> ETGFKCFTCEKAADNYECNRWAPDIYCPRETRYCYTQHTMEVTGNSISVTKRCVPLEECLSTGCR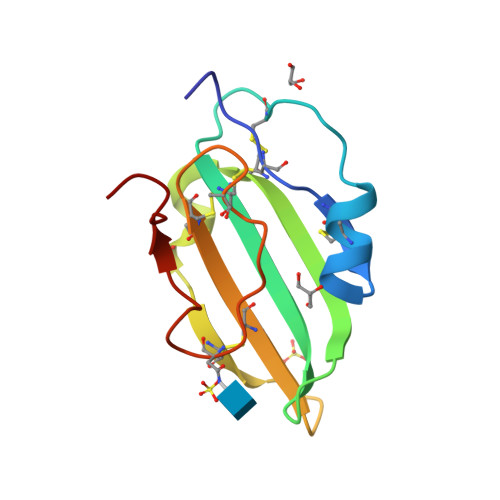DSEHEGHKVCTSCCEGNICNLPLPRNETDATFAGTLEVL dimethyl 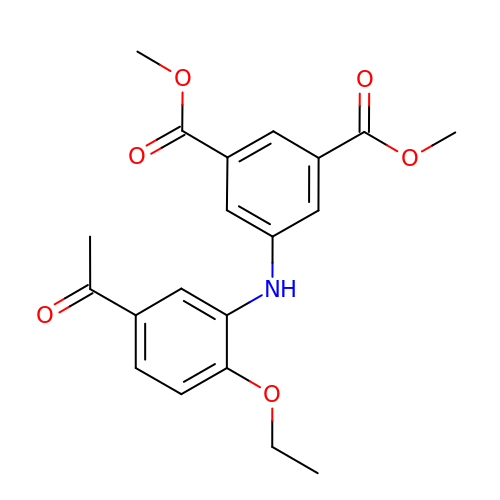5-[(5-ethanoyl-2-ethoxy-phenyl)amino]benzene-1,3-dicarboxylate | C20 H21 N O6 | UNAGVZCODUSBMG-UHFFFAOYSA-N>MKITDLELHAVGIPRHTGFVNKHVIVKIHTDEGLTGIGEMSDFSHLPLYSVDLHDLKQGLLSILLGQNPFDLMKINKELTDNFPETMYYFEKGSFIRNGIDNALHDLCAKYLDISVSDFLGGRVKEKIKVCYPIFRHRFSEEVESNLDVVRQKLEQGFDVFRLYVGKNLDADEEFLSRVKEEFGSRVRIKSYDFSHLLNWKDAHRAIKRLTKYDLGLEMIESPAPRNDFDGLYQLRLKTDYPISEHVWSFKQQQEMIKKDAIDIFNISPVFIGGLTSAKKAAYAAEVASKDVVLGTTQELSVGTAAMAHLGCSLTNINHTSDPTGPELYVGDVVKNRVTYKD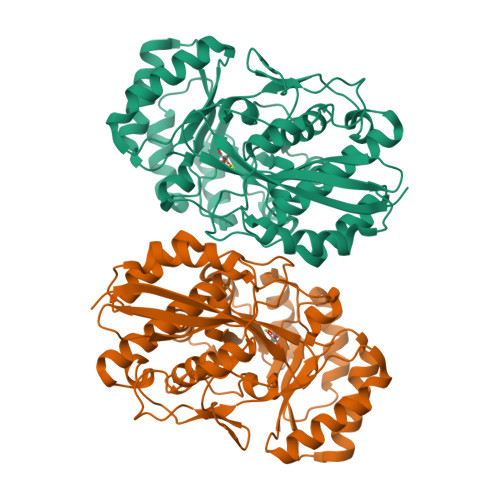GYLYAPDRSVKGLGIELDESLLAKYQVPDLSWDNVTVHQLQDRTADTKS[2x]>[2x]MSENLKDEILEKYIPKTKKTRSGHIVIKTEETPNPEIVANTRTVPGIITARGCAYAGCKGVVMGPIKDMVHITHGPIGCSFYTWGGRRFKSKPENGTGLNFNEYVFSTDMQESDIVFGGVNKLKDAIHEAYEMFHPAAIGVYATCPVGLIGDDILAVAATASKEIGIPVHAFSCEGYKGVSQSAGHHIANNTVMTDIIGKGNKEQKKYSINVLGEYNIGGDAWEMDRVLEKIGYHVNATLTGDATYEK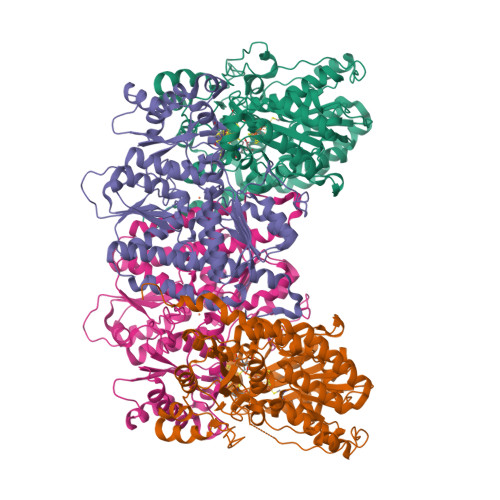VQNADKADLNLVQCHRSINYIAEMMETKYGIPWIKCNFIGVDGIVETLRDMAKCFDDPELTKRTEEVIAEEIAAIQDDLDYFKEKLQGKTACLYVGGSRSHTYMNMLKSFGVDSLVAGFEFAHRDDYEGREVIPTIKIDADSKNIPEITVTPDEQKYRVVIPEDKVEELKKAGVPLSSYGGMMKEMHDGTILIDDMNHHDMEVVLEKLKPDMFFAGIKEKFVIQKGGVLSKQLHSYDYNGPYAGFRGVVNFGHELVNGIYTPAWKMITPPWK;>[2x]MLDATPKEIVERKALRINPAKTCQPVGAMYAALGIHNCLPHSHGSQGCCSYHRTVLSRHFKEPAMASTSSFTEGASVFGGGSNIKTAVKNIFSLYNPDIIAVHTTCLSETLGDDLPTYISQMEDAGSIPEGKLVIHTNTPSYVGSHVTGFANMVQGIVNYLSENTGAKNGKINVIPGFVGPADMREIKRLFEAMDIPYIMFPDTSGVLDGPTTGEYKMYPEGGTKIEDLKDTGNSDLTLSLGSYASDLGAKTLEKKCKVPFKTLRTPIGVSATDEFIMALSEATGKEVPASIEEERGQLIDLMIDAQQYLQGKKVALLGDPDEIIALSKFIIELGAIPKYVVTGTPGMKFQKEIDAMLAEAGIEGSKVKVEGDFFDVHQWIKNEGVDLLISNTYGKFIAREENIPFVRFGFPIMDRYGHYYNPKVGYKGAIRLVEEITNVILDKIERECTEEDFEVVR>[2x]MMAGARRLELGEALALGSGWRHACHALLYAPDPGMLFGRIPLRYAILMQMRFDGRLGFPGGFVDTQDRSLEDGLNRELREELGEAAAAFRVERTDYRSSHVGSGPRVVAH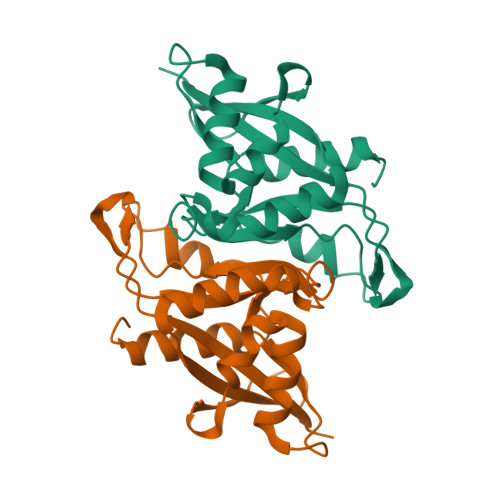FYAKRLTLEELLAVEAGATRAKDHGLEVLGLVRVPLYTLRDGVGGLPTFLENSFIGSAREQLLEALQDLGLLQSGSISGLKIPAHHHHHH>[4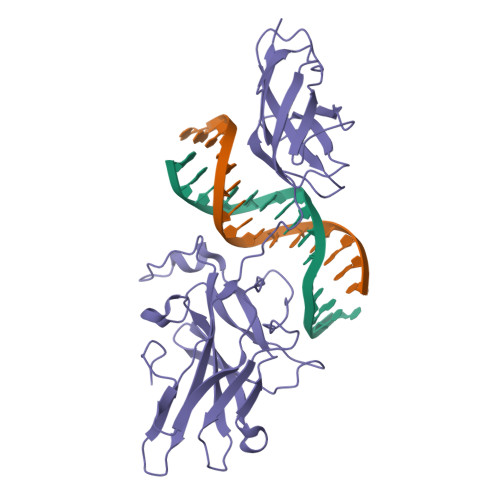x]VPLEWPLSSQSGSYELRIEVQPKPHHRAHYETEGSRGAVKAPTGGHPVVQLHGYMENKPLGLQIFIGTADERILKPHAFYQVHRITGKTVTTTSYEKIVGNTKVLEIPLEPKNNMRATIDCAGILKLRNADIELRKGETDIGRKNTRVRLVFRVHIPESSGRIVSLQTASNPIECSQRSAHELPMVERQDTDSCLVYGGQQMILTGQNFTSESKVVFTEKTTDGQQIWEMEATVDKDKSQPNMLFVEIPEYRNKHIRTPVKVNFYVINGKRKRSQPQHFTYHPV>[2x]GSMTNIPFIYQYEEKENERAAAGYGTFGYLITRIEETL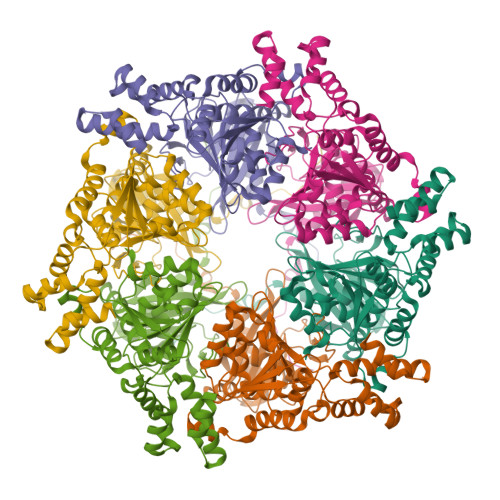YDQYGVFYELYASDDPNTEYWELLVEDVRSGSLEPEHVAYIFEKLEKKTFAYDEDEKEPDYTVHKSIRNSVYAYPEKGVAFARIPYFQDGSIMSFDCLFAVNDEKMRAFLEGVRPRLWEKSKRKVTVFTDGDGGTSREQEAIVREVQRSQVIMNPLLKKEIYRSIDQFFHSDKSFYQTYDIPYKRGILLYGPPGNGKTTLVKSIAGSIDAPVAYWQITEFTSSETIEEVFQAARRLAPAVLVIEDIDSMPEDVRSFFLNTLDGATSKEGLFLIGTTNYPEEIDPGLMNRAGRFDRAYEIGLPDEELRLEYMKMRGFGIFLSEGEIKNAAKLTEGFSFAQLGELYVSSALQWHQEGNHHIETMVKDMTGEQRKSQRGSWMERNKVGFH>[2x]PAKKPLTKIVSHLLVA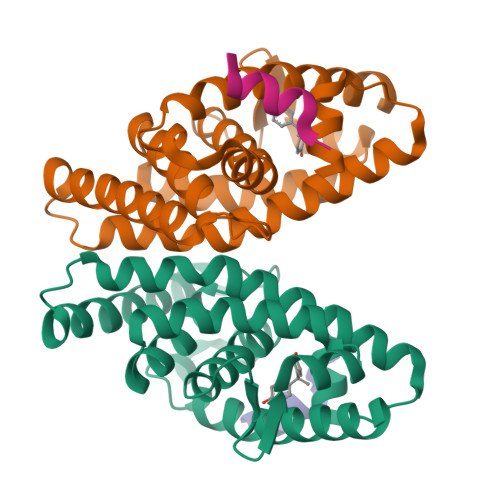EPDKLYAMPPPGMPEGDIKALTTLCDLADRELVVIIGWAKHIPGFSSLSLGDQMSLLQSAWMEILILGIVYRSLPYDDKLVYAEDYIMDEEHSRLAGLLELYRAILQLVRRYKKLKVEKEEFVTLKALALANSDSMHIEDLEAVQKLQDLLHEALQDYELSQHHEEPWRTGKLLLTLPLLRQTAAKAVQHFYSVKLQGKVPMHKLFLEMLEAKV;>[2x]KHKILHRLLQD>[2x]VSEPTTVAFDVRPGGVVHSFSHNVGPGDKYTCMFTYASQGGTNEQWQMSLGTSEDHQHFTCTIWRPQGKSYLYFTQFKAEVRGA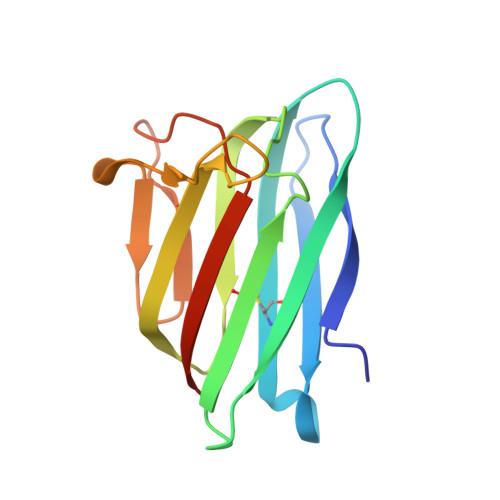EIEYAMAYSKAAFERESDVPLKTEEFEVTKTAVAHRPGAFKAELSKLVIVAKASRTEL>[2x]AQYEDGKQYTTLEKPVAGAPQVLEFFSFFCPHCYQFEEVLHISDNVKKKLPEGVKMTKYHVNFMGGDLGKDLTQAWAVAMALGVEDKVTVPLFEGVQKTQTIRSASDIRDVFINAGIK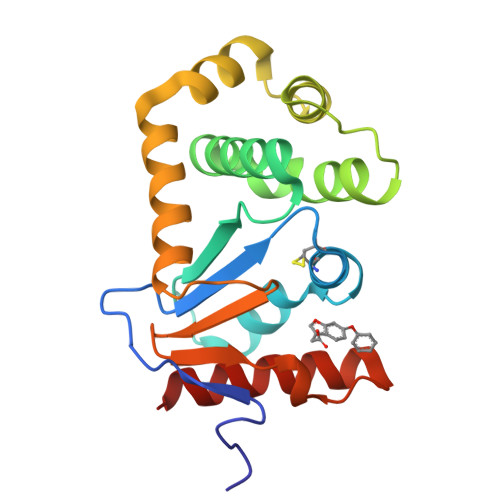GEEYDAAWNSFVVKSLVAQQEKAAADVQLRGVPAMFVNGKYQLNPQGMDTSNMDVFVQQYADTVKYLSEKK> TIARTIVLQESIGKGRFGEVWRGKWRGEEVAVKIFSSREERSWFREAEIYQTVMLRHENILGFIAADNKDNGTWTQLWLVSDYHEHGSLFDYLNRYTVTVEGMIKLALSTASGLAHLHMEIVGTQGKPAIAHRDLKSKNILVKKNGTCCIADLGLAVRHDSA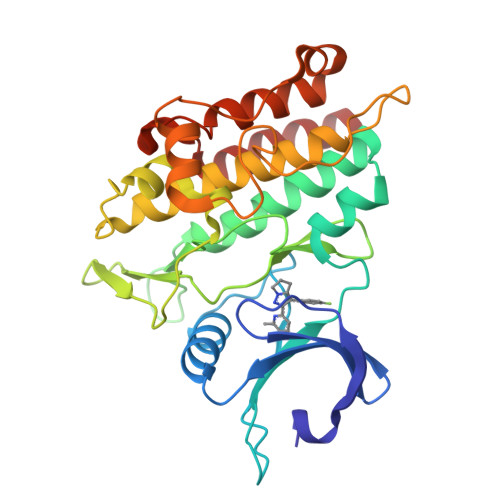TDTIDIAPNHRVGTKRYMAPEVLDDSINMKHFESFKRADIYAMGLVFWEIARRCSIGGIHEDYQLPYYDLVPSDPSVEEMRKVVCEQKLRPNIPNRWQSCEALRVMAKIMRECWYANGAARLTALRIKKTLSQLSQQEG> MGSSHHHHHHSSGRENLYFQGMNNKHATSAVHEIIREICRLVDSGHSMTRDQFHELSEQERFIAFLAEKYSSTIKLYYLADSSPLFEKDTSSFIENAFGRH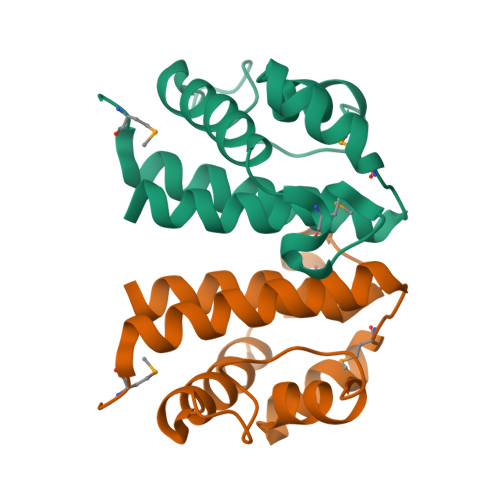ANTVVMEDFGLKSNALLLAINICLAILREINGEV> GPLGSNNVN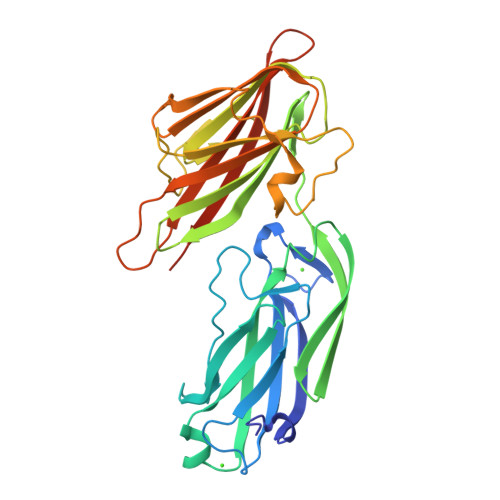DLITVTKQMITEGIKDDGVIQAHDGEHIIYTSDFKIDNAVKAGDTMTVKYDKHTIPSDITDDFTPVDITDPSGEVIAKGTFDLNTKTITYKFTDYVDRYENVNAKLELNSYIDKKEVPNETNLNLTFATADKETSKNVKVEYQKPIVKDESNIQSIFSHLDTTKHEVEQTIYVNPLKLNAKNTNVTIKSGGVADNGDYYTGDGSTIIDSNTEIKVYKVASGQQLPQSNKIYDYSQYEDVTNSVTINKNYGTNMANINFGDIDSAYIVKVVSKYTPGAEDDLAVQQGVRMTTTNKYNYSSYAGYTNTILSTTDSGGGDGTVKP> ELPQMTQQLNSDDMQEQLSATVKFRQILSREHRPPIDVVIQAGVVPRLVEFMRENQPEMLQLEAAWALTNIASGTSAQTKVVVDADAVPLFIQLLYTGSVEVKEQAIWALGNVAGDSTDYRDYVLQCNAMEPILGLFNSNKPSLIRTATWTLSNLCRGKKPQPDWSVVSQALPTLAKLIYSMDTETLVDACWAISYLSDGPQEAIQAVIDVRIPKRLVELLSHESTLVQTPALRAVGNIVTGNDLQTQVVINAGVLPALRLLLSSPKENIKKEACWTISNIT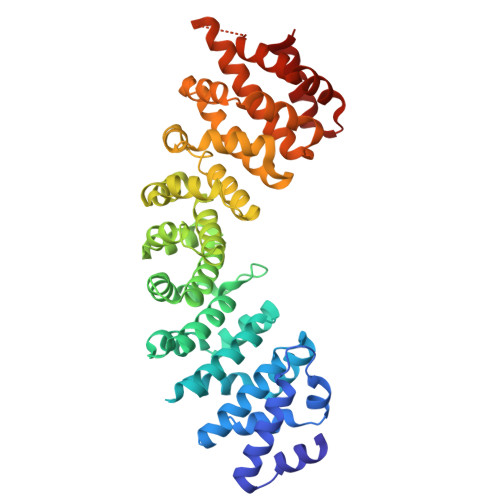AGNTEQIQAVIDANLIPPLVKLLEVAEYKTKKEACWAISNASSGGLQRPDIIRYLVSQGCIKPLCDLLEIADNRIIEVTLDALENILKMGEADKEARGLNINENADFIEKAGGMEKIFNCQQNENDKIYEKAYKIIETYFG GAMMA-BUTYROLACTONE | C4 H6 O2 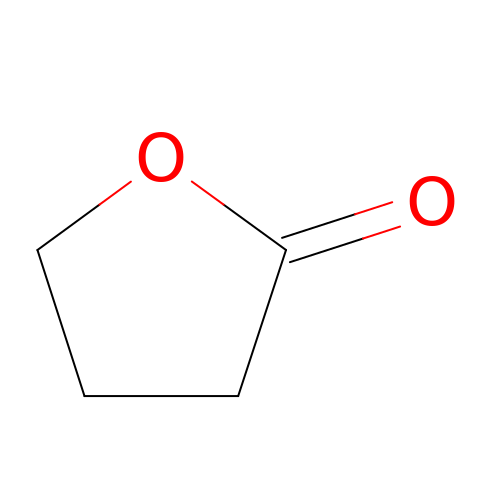| YEJRWHAVMIAJKC-UHFFFAOYSA-N> GDDNNAAEVDRQVAQDSAEPKTGENAAAGDSSSTNKN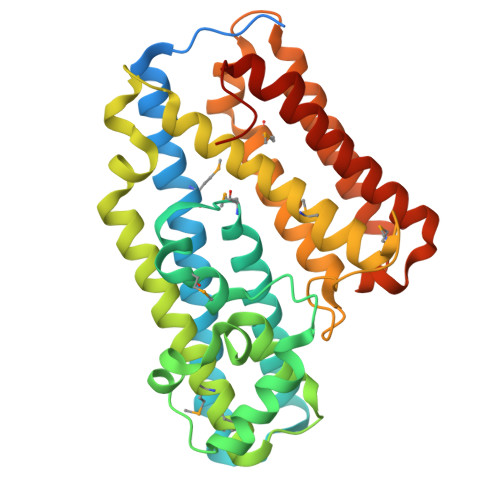AEKIVAVDISAETEKTYLTHVANDMVIPAYADAAKQSDLLHDLAQKHCQKAPVSGDELQALRDQWLVLAQAWASAEMVNFGPATASMSNLYINYYPDERGLVHGGVADLITANPALTAEQLANESAVVQGIPGLEEALYANDSLDAGQCAYVMSASSALGTRLKDIEKNWQQNAIKLLAIDKTAESDQGLNQWFNSLLSLVETMKSNAIEQPLGLSGKAKGHLPAATAGQSRAIINAKLATLNKAMTDPVLTAILGSNNENTVADTLSTALADTTALLAQMPEDLATADKATQQELYDHLTNITRLIKSQLIPTLGIRVGFNSTDGD> MSAVKAARYGKDNVRVYKVHKDEKTGVQTVYEMTVCVLLEGEIETSYTKADNSVIVATDSIKNTIYITAKQNPVTPPELFGSILGTHFIEKYNHIHAAHVNIVCHRWTRMDIDGKPHPHSFIRDSEEKRNVQVDVVEGKGIDIKSSLSGLTVLKSTNSQFWGFLRDEYTTLKETWDRILSTDVDATWQWKNFSGLQEVRSHVPKFDATWATAREVTLKTFAEDNSASVQATMYKMAEQILARQQLIETVEYSLPNKHYFEIDLSWHKGLQNTGKNAEVFAPQSDPNGLIKCTVGRSSLKSKL

Serial crystallography at conventional synchrotron light sources (SSX) offers the possibility to routinely collect data at room temperature using micrometre-sized crystals of biological macromolecules. We show here the versatility of this setup and methodology by performing structural studies at room temperature (RT) of three additional enzyme systems of biological relevance: (i) Klebsiella pneumoniae CTX-M-14 β-lactamase, a β-lactamase relevant to multi-antibiotic resistance mechanisms; (ii) Nectria haematococca xylanase GH11, a highly active xylanase suitable for industrial applications; and (iii) Aspergillus flavus urate oxidase (UOX) in the presence of the long-lived intermediate-like 5-per­oxy-9-methyl-isourate (5PMUA).

Unlike the other experiments discussed here, in the case of the UOX-5PMUA complex no attempt was made to grow microcrystals. Instead, we purposefully crushed twelve large crystals (approximate volume of each crystal 0.13 mm3) using 1 mm-diameter glass beads to explore whether this rather coarse approach could be useful for SSX experiments, for example, when microcrystal optimization is problematic. Overall, this approach afforded, after merging, a complete 2.3 Å resolution dataset that was employed to determine the structure of the UOX-5PMUA complex at RT. UOX crystallizes in space group I222 with one monomer in the crystallographic atomic unit. The tetrameric arrangement with the D 2 point group that constitutes its quaternary structure is generated in the crystal by symmetry. As previously observed in the structure of the complex solved at cryo-temperature, 5PMUA binds at the interface between two protomers of the UOX tetrameric assembly in a cavity lined by K10*, I54*, A56*, T57*, D58*, F159, R176, L170, S226, V227, Q228, N254, H256, G286, I288 (the asterisk indicates residues belonging to a separate UOX chain) with the peroxide moiety sandwiched between the side chains of T57* and N254. The peroxide moiety displays pronounced pyramidalization at C5 accompanied by the strong distortion of its fused heterocycles. The C5—O1 bond length refines at the target value of 1.44 Å with no indication of C5—O1 rupture visible in mF o − DF c maps at the ±3σ level. We find that cell dimensions are modestly affected by cryo-cooling with a unit-cell volume contraction of about 2.1% (a = 79.79/79.51 Å, b = 96.03/95.13 Å, c = 105.21/104.31 Å – RT/100 K). Overall, the present RT medium-resolution complex is virtually identical to that at 100 K and near-atomic resolution with an RMSD of 0.23 Å for all common main-chain atoms in the residue range (1–295) [Fig. 9(a)]. Overall, the quick ‘crush-and-collect’ approach employed here allowed the determination of the RT structure of the UOX-5PMUA complex and the visualization of the radiation-sensitive 5PMUA intermediate at medium resolution.>[2x]MPTKKQKSKSKLKPFFALVRRTNPSYGKLAFALALS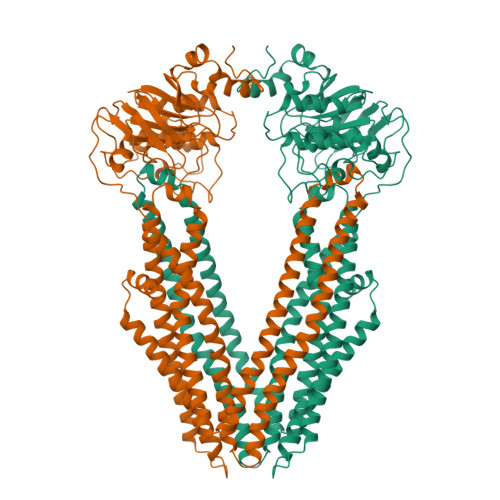VVTTLVSLLIPLLTKQLVDGFSMSNLSGTQIGLIALVFFVQAGLSAYATYALNYNGQKIISGLRELLWKKLIKLPVSYFDTNASGETVSRVTNDTMVVKELITTHISGFITGIISVIGSLTILFIMNWKLTLLVLVVVPLAALILVPIGRKMFSISRETQDETARFTGLLNQILPEIRLVKASNAEDVEYGRGKMGISSLFKLGVREAKVQSLVGPLISLVLMAALVAVIGYGGMQVSSGELTAGALVAFILYLFQIIMPMGQITTFFTQLQKSIGATERMIEILAEEEEDTVTGKQIENAHLPIQLDRVSFGYKPDQLILKEVSAVIEAGKVTAIVGPSGGGKTTLFKLLERFYSPTAGTIRLGDEPVDTYSLESWREHIGYVSQESPLMSGTIRENISYGLERDVTDAEIEKAAEMAYALNFIKELPNQFDTEVGERGIMLSGGQRQRIAIARALLRNPSILMLDEATSSLDSQSEKSVQQALEVLMEGRTTIVIAHRLSTVVDADQLLFVEKGEITGRGTHHELMASHGLYRDFAEQQLKMNCDLENKAGVDKLAAALEHHHHHH> GMGRILREGAGWRLGWDETAHRYPGLVGTTDWAVELTAAEMADFCRLVQQLAETIAAIAPEL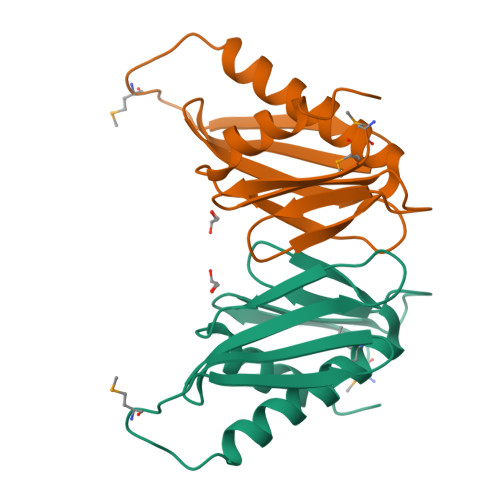MPEERLQIEAESALLWLEAEGFADAYELRLILASDRRVEACWPAAAVPALVAATHTLKGF> MRGSHHHHHHGLVP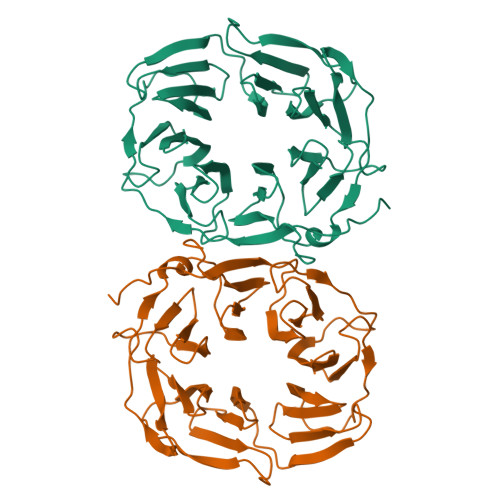RGSAIPALDYNPWEAIQLPTTATILDMSFIDRHHGWLVGVNATLMETRDGGQTWEPRTLVLDHSDYRFNSVSFQGNEGWIVGEPPIMLHTTDGGQSWSQIPLDPKLPGSPRLIKALGNGSAEMITNVGAIYRTKDSGKNWQALVQEAIGVMRNLNRSPSGEYVAVSSRGSFYSTWEPGQTAWEPHNRTTSRRLHNMGFTPDGRLWMIVNGGKIAFSDPDNSENWGELLSPLRRNSVGFLDLAYRTPNEVWLAGGAGALLCSQDGGQTWQQDVDVKKVPSNFYKILFFSPDQGFILGQKGILLRYVTDLTAAPA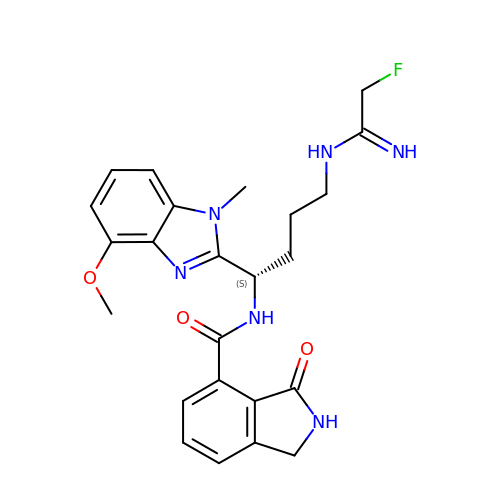~{N}-[(1~{S})-4-(2-fluoranylethanimidoylamino)-1-(4-methoxy-1-methyl-benzimidazol-2-yl)butyl]-3-oxidanylidene-1,2-dihydroisoindole-4-carboxamide | C24 H27 F N6 O3 | DMTSALXYYYZIBF-INIZCTEOSA-N>[4x]MKYILVTGGVISGIGKGIIASSIGTILKSCGLRVTAIKIDPYINIDAGTFSPYEHGEVFVLNDGGEVDLDLGNYERFLDINLYKDNNITTGKIYQHVINKERRGDYLGKTVQVVPHITDAI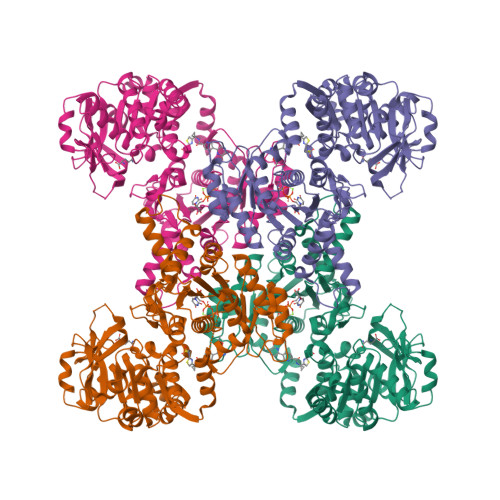QEWVMNQAKVSVDGNKEDPQICVIELGGTIGDIEGMAFVEAFRQFQFKAKKENFYNIHVSLVPQPSATGEQKTKPTQNSVRALRGLGLSPDLIVCRSSTPIEMAVKEKISMFCHVNPEQVICIHDVSSTYRVPLLLEEQGVVKYFQERLGLPINDCSSNLLFKWKAMADRYERLQKICSIALVGKYTKLRDCYASVFKALEHSALAINHKLNLMYIDSIDLEPVTKAEDPVKFHEAWQKLCLADGILVPGGFGIRGTLGKLQAISWARTKKIPFLGICLGMQLAVIEFARNCLNLKDANSTEFEPNTPVPLVIDMPEHNPGDLGGTMRLGLRRTVFTTENSILKKLYGDVPYIEERHRHRYEVNPNLINQFENKDLCFVGEDVDGKRMEIVELTSHPYFIGVQFHPEFSSRPMKPSPPYLGLLLAATGNLNAHLQQMNKLPYSDGYSDASDDSFPEAKLAELDLN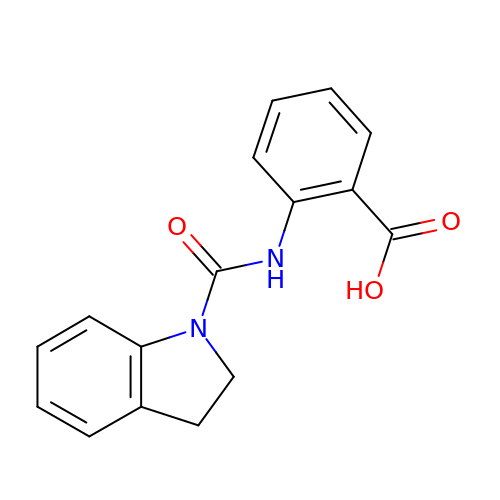2-[(2,3-dihydro-1H-indole-1-carbonyl)amino]benzoic acid | C16 H14 N2 O3 | SEVISWFLUIXPLQ-UHFFFAOYSA-N2-[[3-[[5-(3-iodanylphenyl)carbonylthiophen-2-yl]carbonylamino]phenyl]methyl]propanedioic 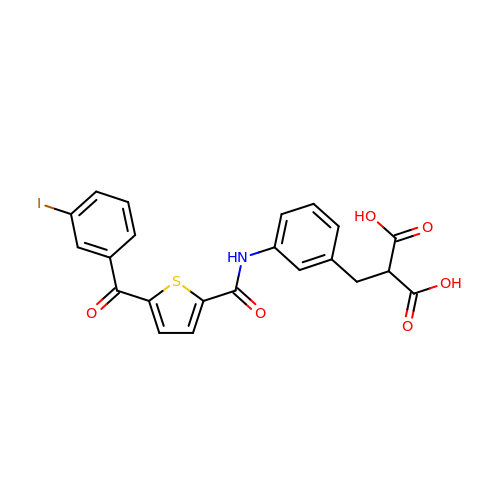acid | C22 H16 I N O6 S | YFWFBHQNVREQSD-UHFFFAOYSA-N>[3x]GHMPEEEKAARLFIEALEKGDPELMRKVISPDTKMVDNGREFTGDEVVEY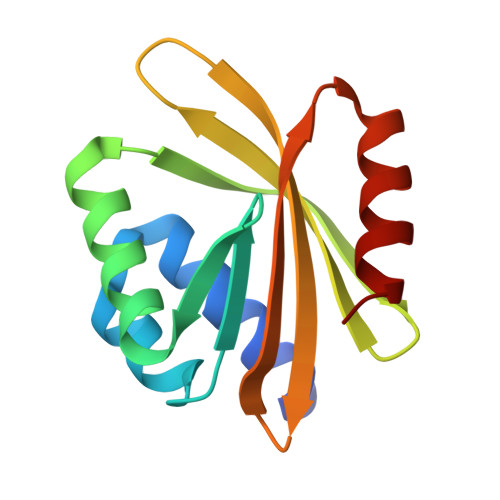VKEIQKRGEQWHLKKYTKIGNVWVFYVQVDNNGQTEIWVVVIKVENGRIKIVFIQTVRDEEEAHEAARKLAKQA>[4x]MGSSHHHHHHSQDLENLYFQGGSTRLSLEAMLAERAMVARQDLAGLKRKLAGADRVLAPQSPEQCGRESAQAQARSVTSELKSAVKEAQGLEHQTLDFLEQLGEYPVCGILHGDHPVHPSGTHNNNGKVSVKRQFAAGVNTSDALTCAFRFEDSDLVRETALKTTYTDGTWAGFVQRLKMQTTRKCVQEKVSRKLLKQLFPYDPQKLVDVSGELSELVLGIKTNAIASAGPPYWRTKRDALPDMLDCVLPLLYDHIVRKDLTTLRNKHPELFLAECKNKTDRYEVESLGEKTRPYFSHPFHLSALVSVLSQSFSGALKIMTEDSTSFNAYGFSWTNGGAEDLAIWARQAGEAGKKPPRIACYGDDTDIYYRKDGKLYRICPDFKQMDGSVDATTIEAVVDYVVDAHVKQYPTARQFWEEVGKLWVEMATQSPFLIDGTKVYRKMQKDGLMTGVVGTTLFDTVKSALAYNDWADQLMFGSLNLLEEKYAIEFFKNKHGLVIKEGTWKPALVNEDPGFGELWTEQKFLGLQLKVVRRENEKVYVPNLPFEDWLTMWVTPRSKYRSKETETMRERTLFDRARGLLVTGAVFDERARGLMGAVINSTAPEVVCMRVQEGGGRGAPPAYAFLTRDGVFEFPISDGYPSYDWVVSLYSRDHPCDMPRVFPEAATLIASYRKQVMDTRVVI

Thosea asigna virus (TaV) is a (+) ssRNA virus that infects the larvae of a defoliating moth (Setothosea asigna) and the prototypic member of the Permutotetraviridae family. In a previous work we have structurally and functionally characterized the non-canonical RdRP domain of TaV (TaVpol: residues 1-674 of the ORF1 product), showing close resemblances with flaviviral RdRPs. In these enzymes, motif C is located upstream of motif A forming a noncanonical C–A–B–D arrangement with a unique connectivity of the major structural elements of the active site. Here we report the X-ray structures of TaVpol captured in three replication-elongation states, revealing high resolution mechanistic details of different events in the nucleotide addition cycle for a non-canonical RdRP.

The incubation of Δ10-TaVpolΔ607-624/5′CAAAAUUU3′/UTP complex cocrystals with Mg2+ resulted in the hydrolysis of the triphosphate molecule, with the incorporation of UMP into the primer molecule in a pretranslocation state. In this state, the 2′-hydroxyl group appeared hydrogen bonded to side chains D447 (motif B) and T438 (motif B), which in turn was bonded to D374 (motif A). Two Mg2+ ions occupied the active site, coordinated by residues Asp369 (motif A), Asp351 (Motif C) and the pyrophosphate (PPi) byproduct. The PPi molecule was also salt bridged by K488 (motif D) and R280 (motif F) in the rNTP tunnel. The newly incorporated uracil (U+1) in this pretranslocation state established a Watson and Crick pair with the A+1 base of the template strand and provided the new 3′ end of the primer terminus. In this state, the conserved catalytic residues D351 (Motif C) and D369 (motif A) still remained coordinated with the two Mg2+ ions. The position B Mg2+ in turn coordinated the ppi byproduct in the rNTP channel. The conserved residues R280 (motif F) and K488 (motif D) were bound the ppi molecule, opposite to metal ions. Another difference between the elongation complexes of TaVpol compared to those of enteroviruses is that the active site closure takes place on RNA template-primer binding, before rNTP binding and is maintained during rNTP recognition but also immediately after nucleotide incorporation.>[2x]GSWFFGKI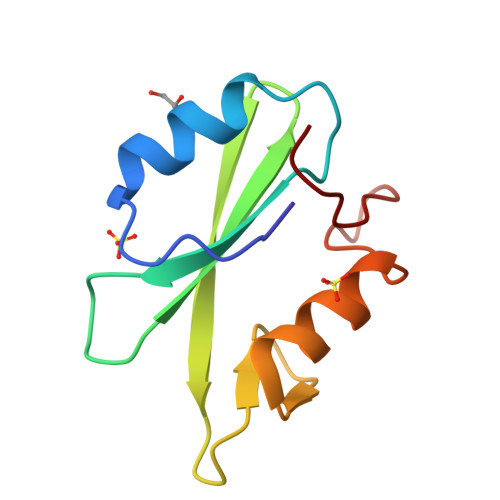PRAKAEEMLSKQRHDGAFLIRESESAPGDFSLSVKFGNDVQHFKVLRDGAGKYFLWVVKFNSLNELVDYHRSTSVSRNQQIFLRDIE> GEEKKDSKAFIDVSAATLWTAPDSLRPIDVPSATNPVDLWKWTKSMTLDEKLWLTNANKLETQALLGQEVTVVDKKGDWVKVLVHGQPTPRNEEGYPGWMPEKQLTYNQEFADKTNEPFVLVTKPTAILYINPSEKHKSLEVSYNTRLPLLSEDTISYRVLLPNGQKAWLRKNDGTFYRSQNDIPTPAADDLINTGKMFLGLPYIWAGTSGFGFDCSGFTHTIYKSHGITIPRDSGPQSRNGVAVDKEHLQKGDLIFFAHDQGKGSVHHVAMYIGDGNMIHSPRAERSVEIIPLNTPGYIEEYAGARRYLP

The crystal structure of a YkfC ortholog from Bacillus cereus (BcYkfC) at 1.8 Å resolution revealed that it contains two N-terminal bacterial SH3 (SH3b) domains in addition to the C-terminal catalytic NlpC/P60 domain that is ubiquitous in the very large family of cell-wall-related cysteine peptidases. NlpC/P60 is a large family of cell-wall related cysteine peptidases that are broadly distributed in bacteria, viruses, archaea and eukaryotes. Characterized NlpC/P60 enzymes are almost all γ-d-Glu-DAP (or γ-d-Glu-Lys) endopeptidases. The first SH3b domain plays an important role in defining substrate specificity by contributing to the formation of the active site, such that only murein peptides with a free N-terminal alanine are allowed.

Here, we report the crystal structure of YkfC from B. cereus (BcYkfC) in complex with l-Ala-γ-d-Glu. The final model of BcYkfC contains residues 29–333, one dipeptide l-Ala-γ-d-Glu, one phosphate, six polyethylene glycol (PEG) fragments from the crystallization solution and 265 waters. The three domains of BcYkfC are arranged in a triangle such that each domain interacts with the two other domains. The active site is located at this SH3b1–NlpC/P60 interface, whereas the SH3b2 domain is distal to the active site. The catalytic triad of the peptidase domain consists of Cys238, His291 and His303. Since an oxidized cysteine can no longer function as a nucleophile in the reaction, the enzyme in the crystal is inactive. As the dipeptide was not added during protein purification or crystallization, it was most likely to have been obtained during protein expression in E. coli. Since this dipeptide is one of the reaction products of BcYkfC, it unequivocally identifies the S2–S1 binding-site cavity, which is formed by residues from both the SH3b1 (Glu83, Thr84 and Tyr118) and NlpC/P60 domains (Tyr226, Trp228, Ala229, Asp237, Arg255, Asp256, Ser257, His290 and His291). The dipeptide is stabilized by multiple hydrogen bonds. The free amine of l-Ala in the S2 pocket makes hydrogen bonds to Glu83 O and the side chains of Tyr118 (OH) and Asp256 (Oδ1), which are highly conserved in the YkfC subfamily of NlpC/P60 enzymes (see below). The l-Ala methyl side chain points towards a hydrophobic pocket defined by the side chains of Trp228 and Ala229.>MPDEEKLQKYLRKVTAELQQARRRLAAAESQSQEPIAVLGIGCRFPGGVRSPEDLWDLVDSGGDAVGGLPAGRGWQAGSALDGVNAGFIHGVEEFDPYFFGLDPVEAAAMDPQQRLLLETTWEAFERAGIDPVAARGSRTAVYAGVQFGGYPLLMREAPPPQVLDHLGLGNSVGAASGRLAYQFGLLGGAVTVDTQCTSSIVALHLAVKALRNGECALALAGGACVMSLPTVLMDFHRRSLLAPDGRSKSFAAAADGVSLAEGAGMLLLERLSDARRNGHPVMAVIRGTAINQDGATNGIISPSGRAQERVIRAALADGRVTADSVDAVEGHGVGATLGDGVEVTSLLSTYGQERPAGRPLLLGSVKSNIGHTQTVGAVAGIVKLVMALRNERLPRTVHVDGPTPHADWSSGTVRLLTEPEPWRRGERVRRAGLTCLTLSGTNGHLILEEPPADEPAARPANPERTVPLVLSAKSPTALREQAERLRATITAAEPVDVGHSLHTTRSSFRHRAVVLGTGREELAAGLDALAGDRTADGLVRGVARAQGQTALLFGGAGDGTSGDRPADAEGPRTARGLYEAFPAFAEALDEVTEHLAGLLGPEVRAAVREPGPACAEPTVVGQAVAFALNTALHRLLTAFAVRPDATLGHGAGEVAAAYAAGALSLADGAALVTALGRITERVATGPGASVWVRATEDEVRAALSGSQEQVGAAVAAVDEPGTTVVSGDAGAVARVAAHWRAHGRATGAPRPARLLLSPDDEQAALAELRAIVAGLAFREPEVPLLSTVTGQPVEPAELRSAEHWLDHLRGPTRFLDGVRRLRTDGVTRLVGLDLSGDLTGPAGRSAAGFGEPGRPLLLASVPGGGRPPGQALLSALGELHTDGVAIDWSQAFEGRGARRVDLPTYPYQKVRCWLVPPEPQVSVVAAPPHPLLGTALDLVDATGQSFTQQLTPGQVAGVFGQQLYGTPVLPAGARLEWLLAAARHGSPDSAWTLTGIRLPGTVSAASGTPVALQTSREDSGDGHRVRAFVKGPGTGGGRWAERGGATVVPAVTRPAPDRVDPESLPEGLAELDVAEVYRRLWRQGSDYAEPLRVLRRVWLGGDEAVALVGTADVPTGPSGWSRWAAVLEAAVQLAALSGSGPRTPVSVDRLEVSGPPSEVVWLRVRHGADGAADAVVLSGEGVRLAAVQGLRLRPMAGREPAGLAEAPLERHEVVWHALAEDGRPGAIGGGTGSWLVFSDDPERAAAWCDELALFGVPAVALAGEDAEGRDGTETVPVGTGDPDVVGKTFAELRERGVTVAGLLVHDAGDAREPASGADDPLDAACRRGGRTLALVRGFLQEYAEQTPRIVLCSAGAAAGLAGGPPHPAQAPLTALFTSLVWEHPELPCAQVDLDPAEDPPTVVSLLGQVMRLPGAGRLAVRGGRWFEARLERRPAPADRGERLALRPDATYLVAGGDTRHAAAALEWLAARGARSVVLAGAESERGDLAGARTTGHAGIERLEHVAVDLSSAADVARLAELCADGRPPLRGVLLLPQPVAGGGLDELDGARFGAELAGALRGPVELTRRFTDVGLTGGTDFFVLSTSVVSLPGRAGTVVGSAADAFLTALARHHRQAGLPVVAAAWGPWLESVDESDEAPAVAFAEAGVYPAPGGEMLDALLPLPAAGEADGSGEAGLARVDWDRYLTAGHRPLPYT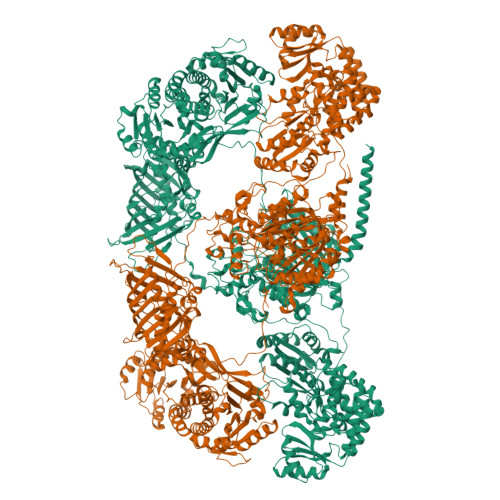VLETRASYDEEKAPGFGQNRMKGARKKKGAAALEHHHHHH[2x]>MVFNLKYTVEEELRAGTKIANVTADAKVAGFALGNRQPYLRVISNSEPRWVNLSPAGLLITKQKIDRDAVCRQTPKCFISLEVMSNSMEICVIKIEIIDVNDNAPRFPTNHIDIEISENAAPGTRFPLEGASDPDSGSNGIQTYTITPNDIFGLEIKTRGDGSKIAELVVEKTLDRETQSRYTFELTAEDGGDPPKSGTVQLNIKVIDSNDNNPVFDEPVYTVNVLENSPINTLVIDLNATDPDEGTNGEVVYSFINFVSNLTKQMFKIDPKTGVITVNGVLDHEELHIHEIDVQAKDLGPNSIPAHCKVIVNVIDINDNAPEIKLLSENSEMVEVSENAPLGYVIALVRVSDNDSG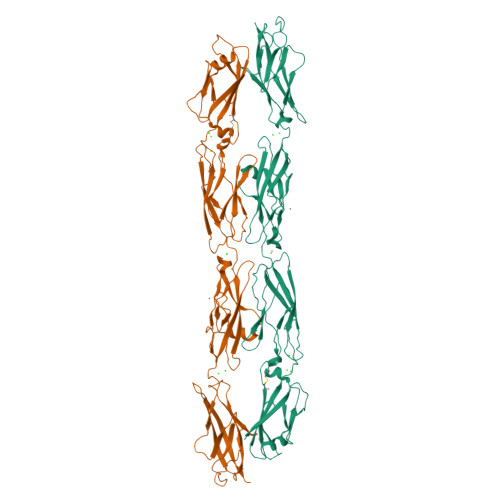ANGKVQCRLQGNVPFRLNEFESFSTLLVDGRLDREQRDMYNLTILAEDSGYPPLRSSKSFAVKVTDLEHHHHHH[2x]>[2x]EIGTGFPFDPHYVEVLGSRMHYVDVGPRDGTPVLFLHGNPTSSYLWRNIIPHVAPSHRCIAPDLIGMGKSDKPDLDYRFDDHVRYLDAFIEALGLEEVVLVIHDWGSALGFHWAKRNPERVKGIAFMEFIRPIPTWDEWPEFARELFQAFRTPDVGRELIIDQNAFIEGILPKFVVRPLTEVEMDHYREPFLKPVWREPLWRFPNELPIAGEPANIWALVEAYMNWLHQSPVPKLLFWGTPGVLIPPAEAARLAESLPNLKTVFIGPGLHYLQEDNPDLIGSEIARWLPAL

Haloalkane dehalogenases (HLDs; EC 3.8.1.5) are α/β-hydrolases that catalyze the hydrolytic cleavage of the carbon–halogen bond in diverse halogenated aliphatic hydrocarbons via SN2 nucleophilic substitution. Structurally, HLDs consist of a canonical α/β-hydrolase fold, which is composed of a central eight-stranded β-sheet domain surrounded by several α-helices (i.e. αβα sandwich architecture). In all HLDs, the active site is positioned in a hydrophobic pocket buried between the α/β-fold core and the cap domain, and this catalytic center is connected with the bulk solvent via a main tunnel and a slot tunnel. After several iteration cycles, we obtained an 11-point DhaA mutant, hereafter referred to as DhaA115, with outstanding thermostability (Tm = 73.5 °C) and thermophilicity, as demonstrated by a substantial shift in the optimal catalytic temperature (Topt = 65 °C).

Here, we report X-ray structures of DhaA115 at 1.55 Å and 1.6 Å resolutions and their molecular dynamics trajectories, which unravel the intricate network of interactions that reinforce the αβα-sandwich architecture. Unexpectedly, mutations toward bulky aromatic amino acids at the protein surface triggered long-distance (∼27 Å) backbone changes due to cooperative effects. These cooperative interactions produced an unprecedented double-lock system that: (i) induced backbone changes, (ii) closed the molecular gates to the active site, (iii) reduced the volumes of the main and slot access tunnels, and (iv) occluded the active site. Despite these spatial restrictions, experimental tracing of the access tunnels using krypton derivative crystals demonstrates that transport of ligands is still effective. Interestingly, despite the active site occlusion, experimental mapping of the enzyme tunnels by krypton derivatization of the DhaA115 crystals, supported by protein dynamics simulations, showed that ligand molecules can still be transported through the enzyme tunnels. Experimental tracking of the tunnels by krypton-derivatization of DhaA115 crystals, supported by protein simulations, revealed that ligands can still be transported through the tunnels as they can open to a significant extent. We expect that this tunnel opening will be even more pronounced at higher temperatures, which would explain the shift in the temperature optimum to a higher range.>[2x]MTQDASPILTSLLDTDAYKLHMQQAVFHHYRHITVAAEFRCRSDELLGVYADEIRHQVTLMGQLALTSDEFIYLSSLPFFQDDYLHWLRDFRFKPEQVSVAVHDGKLDIRIAGLWCEVIMWEVPLLAVISEIVHRRRSTQVTTDQAVQQLRTKLEQFNALSADID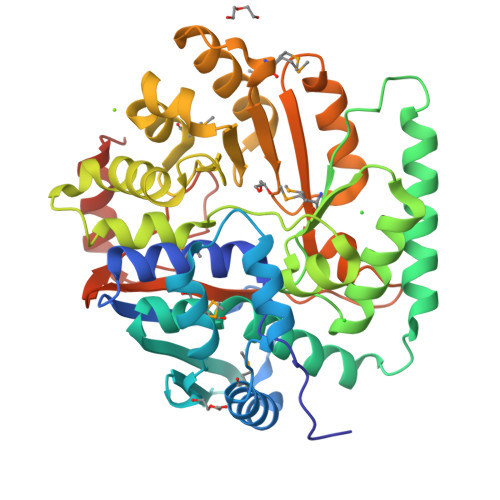ITHFKLMDFGTRRRFSREIQHTVVSTLKDEFPYLVGTSNYDLARTLALAPVGTQAHEWFQAHQQISPTLANSQRVALQVWLDEYPNQLGIALTDCITMDAFLRDFDLAFANRYQGLRHDSGDPIEWGEKAIAHYEKLGIDPMKKVLVFSDNLDLEKALFLYRHFYQRIKLVFGIGTRLTCDIPDVKPLNIVIKLVECNDKPVAKLSDSPGKTICQDPAFVDQLRKAFALPLVKKASENLYFQ> SSPGKPPRLVGGPMDASVEEEGVRRALDFAVGEYNKASNDMYHSRALQVVRARKQIVAGVNYFLDVEVGRTTCTKTQPNLDNCPFHDQPHLKRKAFCSFQIYAVPWQGTMTLS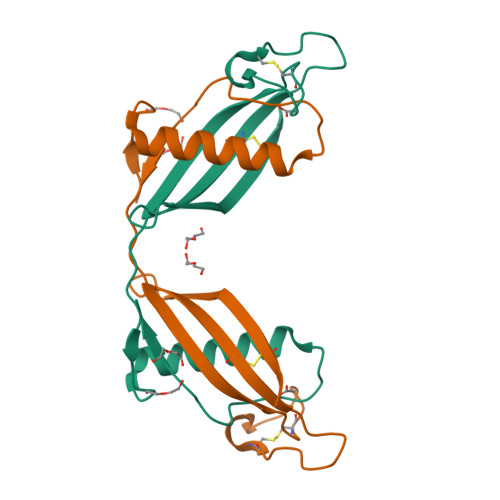KSTCQDA> MQAFGVLDRYIGKTIFNTIMMTLFMLV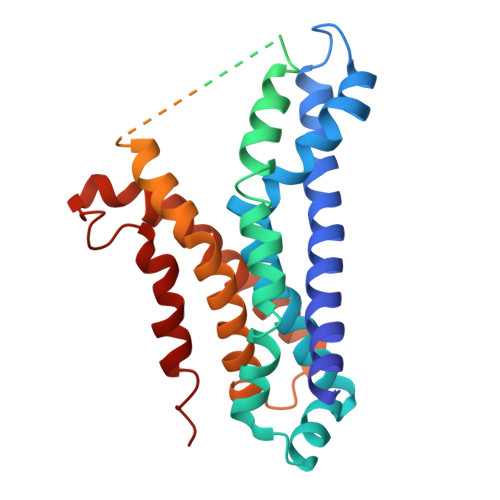SLSGIIKFVDQLKKSGQGSYDALGAGLYTILSVPKDIQIFFPMAALLGALLGLGMLAQRSELVVMQASGFTRLQVALAVMKTAIPLVLLTMAIGEWVAPQGEQMARNYRAQQMYGGSLLSTQQGLWAKDGHNFVYIERVKGNDELGGVSIYAFNPERRLQSVRYAASAKFDSENKVWRLSQVDESDLTDPKQVTGSQMVSGTWKTNLTPDKLGVVALDPDALSISGLHNYVKYLKSSGQDPGRYQLNMWSKIFQPLSVAVMMLMALSFIFGPLRSVPMGVRVVTGISFGFIFYVLDQIFGPLTLVYGIPPIIGALLPSASFFLISLWLMMRKA>SNAMKFLVTGAAGFIGFHIAQRLLNEGHNVVGIDNMNDYYDVSLKQARLDRLAYPAFHFQQLDLADREGMAKLFATEQFDRVIHLAAQAGVRYSLENPYAYADANLMGYLNILEGCRHTKVKHLVYASSSSVYGLNRKMPFSTEDSVDHPVSLYAATKKANELMAHTYSHLYGIPTTGLRFFTVYGPWGRPDMALFKFTKAMLEGKSIDVYNYGKMKRDFTYIDDIVEAVVRVLDVIPQANAD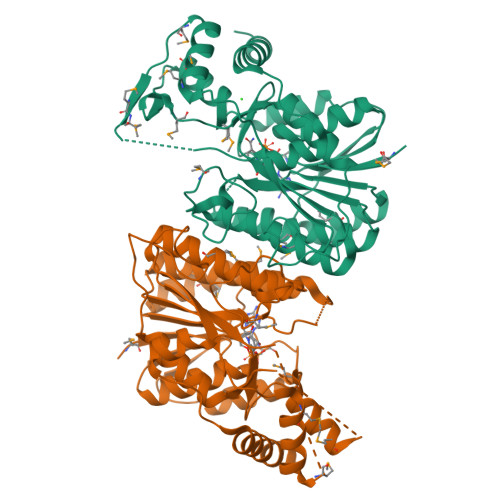WTVESGSPATSSAPYRVYNIGNSSPVELMDYITALEEALGMEAQKNMMPIQPGDVLDTSADTQPLYDLVGFKPQTSVKDGVKNFVDWYKDYYQI[2x]> MTVRYDILPLSPVSRNRLAQVKRKILVLDLDETLIHSHHDGVLRPTVRPGTPPDFILKVVIDKHPVRFFVHKRP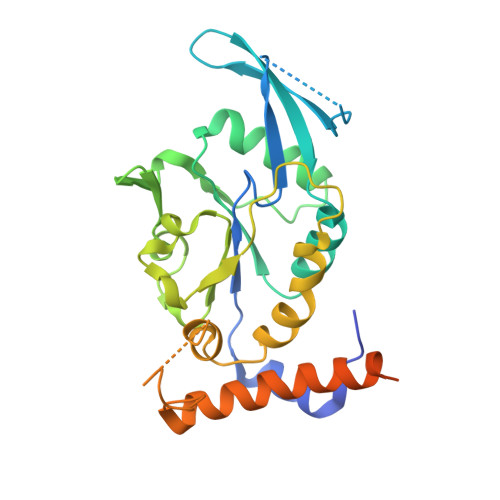HVDFFLEVVSQWYELVVFTASMEIYGSAVADKLDNSRSILKRRYYRQHCTLELGSYIKDLSVVHSDLSSIVILDNSPGAYRSHPDNAIPIKSWFSDPSDTALLNLLPMLDALRFTADVRSVLSRNLHQHRLWGSAKGSESNSLEQAEDLKAFERRLTEYIHCLQAPSIIAARCRTVLAEYNMSCDDTGKLILKPRPHHHHHH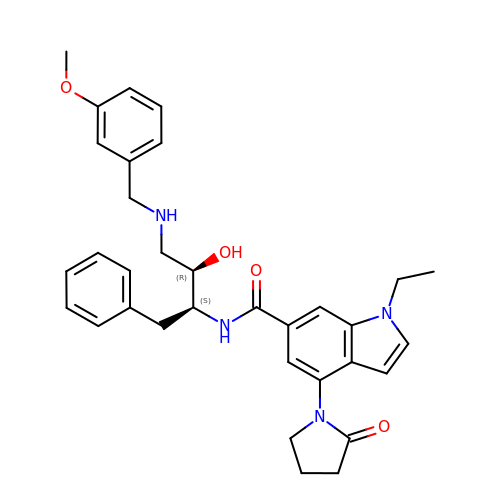N-{(1S,2R)-1-BENZYL-2-HYDROXY-3-[(3-METHOXYBENZYL)AMINO]PROPYL}-1-ETHYL-4-(2-OXOPYRROLIDIN-1-YL)-1H-INDOLE-6-CARBOXAMIDE | C33 H38 N4 O4 | BARAICYUEPEIRD-QCENPCRXSA-N> MRPALYFCGSIRGGREDRTLYERIVSRLRRFGTVLTEHVAAAELGARGEEAAGGDRLIHEQDLEWLQQADVVVAEVTQPSLGVGYELGRAVAFNKRILCLFRPQSGRVLSAMIRGAADGSRFQVWDYEEGEVEALLDRYFEADPLEENL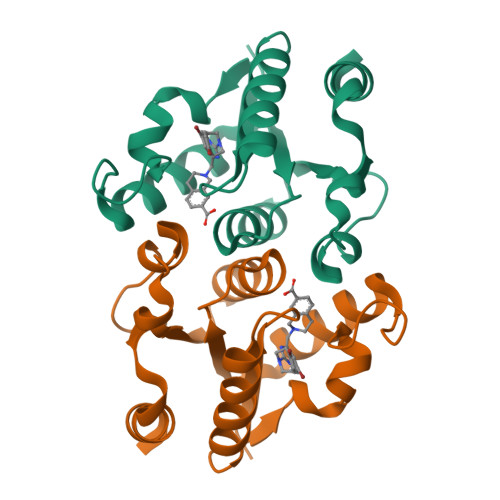YFQ>[4x]SPLAAYEVDDSTGYLTSDVGGPIQDQTSLKAGIRGPTLLEDFMFRQKIQHFDHERVPERAVHARGAGAHGTFTSYADWSNITAASFLNATGKQTPVFVRFSTVAGSRGSADTARDVHGFATRFYTDEGNFDIVGNNIPVFFIQDAIQFPDLIHSVK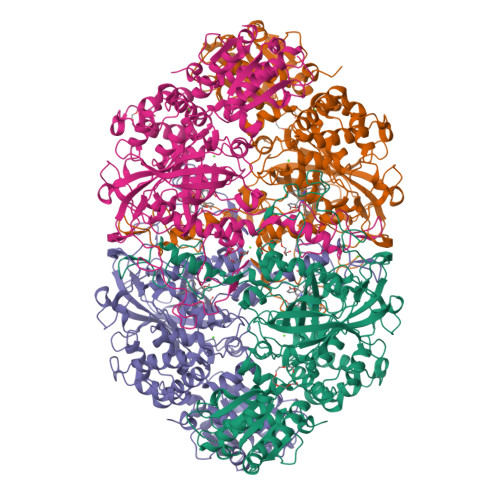PRPDNEIPQAATAHDSAWDFFSQQPSTMHTLFWAMSGHGIPRSYRHMDGFGIHTFRFVKDDGSSKLIKWHFKSRQGKASLVWEEAQVLSGKNADFHRQDLWDAIESGNGPEWDVCVQIVDESQAQAFGFDLLDPTKIIPEEYAPLTKLGLLKLDRNPTNYFAETEQVMFQPGHIVRGIDFTEDPLLQGRLFSYLDTQLNRNGGPNFEQLPINMPRVPIHNNNRDGAGQMFIHRNKYPYTPNTLNSGYPRQANQNAGRGFFTAPGRTASGALVREVSPTFNDHWSQPRLFFNSLTPVEQQFLVNAMRFEISLVKSEEVKKNVLTQLNRVSHDVAVRVAAAIGLGAPDADDTYYHNNKTAGVSIVGSGPLPTIKTLRVGILATTSESSALDQAAQLRTRLEKDGLVVTVVAETLREGVDQTYSTADATGFDGVVVVDGAAALFASTASSPLFPTGRPLQIFVDAYRWGKPVGVCGGKSSEVLDAADVPEDGDGVYSEESVDMFVEEFEKGLATFRFTDRFALDS> MSKEIPTPYMWSYQPQMGLAAGASQDYSTRMNWLSAG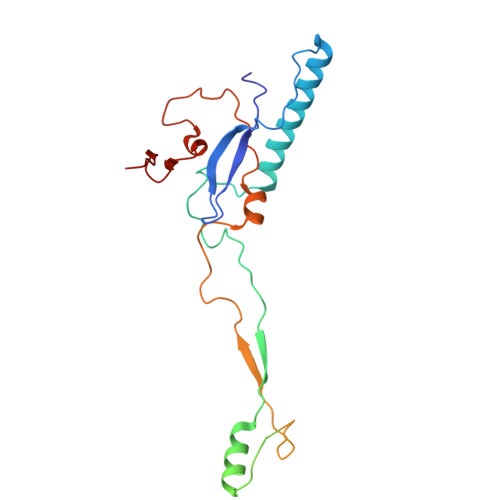PSMISRVNGVRNHRNQILLEQAAVTSTPRAKLNPRNWPSTLVYQEIPGPTTVLLPRDALAEVRMTNSGVQLAGGASRCPLRPQSGIKTLVIRGRGTQLNDELVSSSIGLRPDGVFQLAGAGRSSFTPNQAYLTLQSSSSEPRSGGIGTLQFVEEFVPSVYFNPFSGSPGLYPDEFIPNFDAVREAVDGYD o-succinylbenzoyl-N-coenzyme A | C32 H45 N8 O20 P3 | 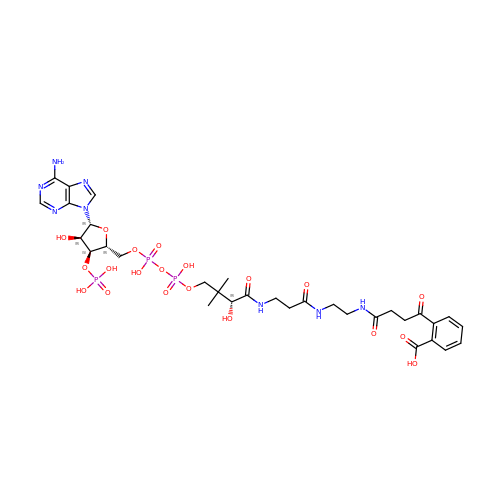QCTNXUGGWNSKFY-HSJNEKGZSA-N> GA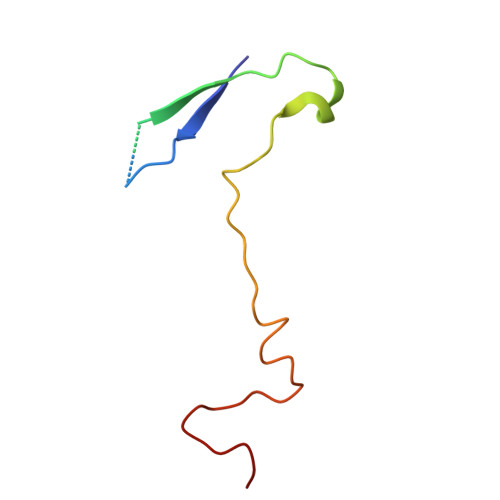QVSTQKTGAHETSLNAAGNSVIHYTNINYYKDAASNSANRQDFTQDPGKFTEPVKDIMVKSMPALN>MSNETLSADVVIIGAGICGSLLAHKLVRNGLSVLLLDAGPRRDRSQIVENWRNMPPDNKSQYDYATPYPSVPWAPHTNYFPDNNYLIVKGPDRTAYKQGIIKGVGGTTWHWAASSWRYLPNDFKLHSTYGVGRDYAMSYDELEPYYYEAECEMGVMGPNGEEITPSAPRQNPWPMTSMPYGYGDRTFTEIVSKLGFSNTPVPQARNSRPYDGRPQCCGNNNCMPICPIGAMYNGVYAAIKAEKLGAKIIPNAVVYAMETDAKNRITAISFYDPDKQSHRVVAKTFVIAANGIETPKLLLLAANDRNPHGIANSSDLVGRNMMDHPGIGMSFQSAEPIWAGGGSVQMSSITNFRDGDFRSEYAATQIGYNNTAQNSRAGMKALSMGLVGKKLDEEIRRRTAHGVDIYANHEVLPDPNNRLVLSKDYKDALGIPHPEVTYDVGEYVRKSAAISRQRLMDIAKAMGGTEIEMTPYFTPNNHITGGTIMGHDPRDSVVDKWLRTHDHSNLFLATGATMAASGTVNSTLTMAALSLRAADAILNDLKQG[2x];>MEKIADSGPVQIFLSRRKLLAFSGASLTVAAIGAPSKGSTQDVVASNRDSISDFMQLSAFATGHKNLDLNIGSALLLAFEAQKHDFSTQIKALREHITKNNYQDVEALDAAMKDDPLHPTLIQIIRAWYSGVIEDETNAKVYAFEKALMYQPSRDVVVIPTYAHNGPNYWVSEPAS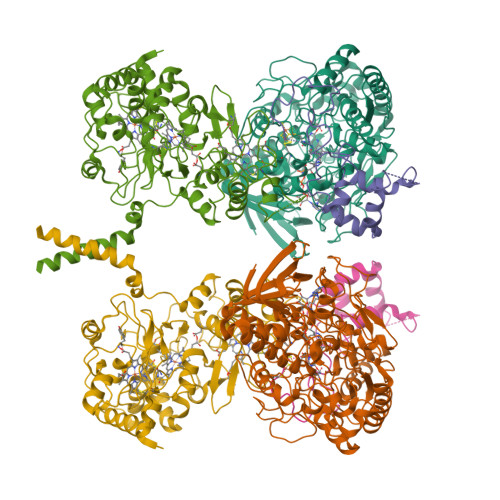VDVMPAF[2x];>[2x]MRYFRPLSATAMTTVLLLAGTNVRAQPTEPTPASAHRPSISRGHYLAIAADCAACHTNGRDGQFLAGGYAISSPMGNIYSTNITPSKTHGIGNYTLEQFSKALRHGIRADGAQLYPAMPYDAYNRLTDEDVKSLYAYIMTEVKPVDAPSPKTQLPFPFSIRASLGIWKIAARIEGKPYVFDHTHNDDWNRGRYLVDELAHCGECHTPRNFLLAPNQSAYLAGADIGSWRAPNITNAPQSGIGSWSDQDLFQYLKTGKTAHARAAGPMAEAIEHSLQYLPDADISAIVTYLRSVPAKAESGQTVANFEHAGRPSSYSVANANSRRSNSTLTKTTDGAALYEAVCASCHQSDGKGSKDGYYPSLVGNTTTGQLNPNDLIASILYGVDRTTDNHEILMPAFGPDSLVQPLTDEQIATIADYVLSHFGNAQATVSADAVKQVRAGGKQVPLAKLASPGVMLLLGTGGILGAILVVAGLWWLISRRKKRSA>[4x]MHHHHHHGKNHAGSPGCEESAAGKEKLPKMRLPTRSDMICGYACLKGTAAMRNTKRGSWYIEALAQVFSERA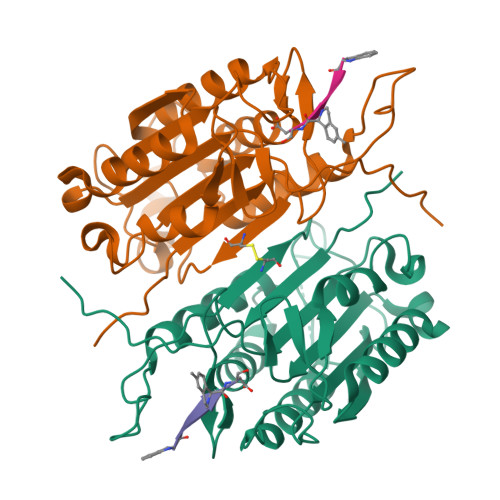CDMHVADMLVKVNALIKDREGYAPGTEFHRCKEMSEYCSTLCRHLYLFPGGGVKPCTPEFYQTHFQLAYRLQSRPRGLALVLSNVHFTGEKELEFRSGGDVDHSTLVTLFKLLGYDVHVLCDQTAQEMQEKLQNFAQLPAHRVTDSCIVALLSHGVEGAIYGVDGKLLQLQEVFQLFDNANCPSLQNKPKMFFIQACRGDETDRGVDQQD>[4x]MDTNKREIVEFLGIRTYFFPNLALYAVNNDELLVSDPNKANSFAAYVFGASDKKPSVDDIVQMLFPSGSDSGTILTSMDTLLALGPDFLTEFKKRNQDLARFNLTHDLSILAQGDEDAAKKKLNLMGRKAKLQKTEAAKILAILIKTINSEENYEKFTELSELCGLDLDFDAYVFTKILGLEDEDTADEVEVIRDNFLNRLDQTKPKLADIMRNGP

Two PGL proteins, PGL-1 and PGL-3, are key scaffolding proteins required for proper P granule assembly. PGL proteins can self-assemble into granules, both in vitro using purified recombinant protein9,11,12 and in intestinal nematode cells or mammalian cells in culture when expressed on their own. These in vitro PGL granules display liquid droplet behavior, indicating that PGL protein alone is sufficient to recapitulate the biophysical properties of P granules in nematode cells. Assays for granule assembly in mammalian cells implicated the conserved N-terminal region of PGL as critical, and structural studies identified a central dimerization domain (DD) within that conserved region.

The NtDD has a novel fold consisting of 11 alpha helices and a single N-terminal beta strand. While each ASU possessed two pairs of identical interfaces, one of these interface pairs consisted of a network of conserved amino acid side chains making extensive salt bridges and hydrogen bonds. The complexity and conservation of these interactions suggested biological relevance. We conclude that the dimers observed in the crystal structure represent the NtDD dimer detected in solution.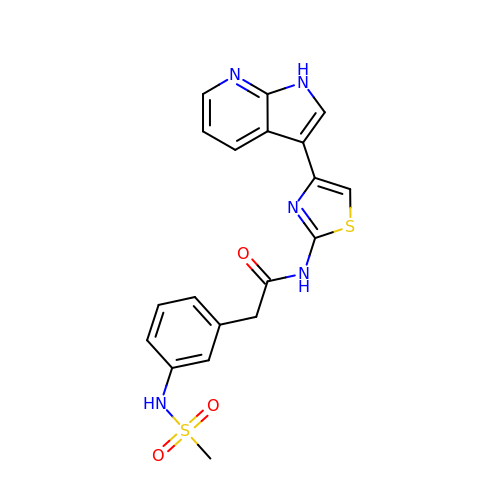2-[3-(methylsulfonylamino)phenyl]-~{N}-[4-(1~{H}-pyrrolo[2,3-b]pyridin-3-yl)-1,3-thiazol-2-yl]ethanamide | C19 H17 N5 O3 S2 | HIUHVDROHDSKTC-UHFFFAOYSA-N> GSHMAKYTREDIEKLVKEENVKYIRLQFTDILGTIKNVEIPVSQLGKALDNKVMFDGSSIEGFVRIEESDMYLYPDLNTFVIFPWTAEKGKVARFICDIYNPDGTPFEGDPRNNLKRILKEMEDLGFSDFNLGPEPEFFLFKLDEKGEPTLELNDKGGYFDLAPTDLGENC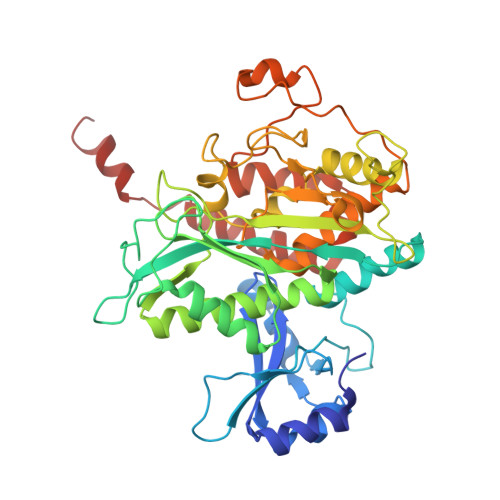RRDIVLELEEMGFEIEASHHEVAPGQHEIDFKYAGAVRSCDDIQTFKLVVKTIARKHGLHATFMPKPLFGVNGSGMHCNLSLFKNGVNAFFDENADLQLSETAKHFIAGIVKHATSFTAVTNPTVNSYKRLVPGYEAPCYVAWSAQNRSPLIRIPASRGISTRVEVRSVDPAANPYLALSVLLAAGLDGIKNKLEAPAPIDRNIYVMSKEERMENGIVDLPATLAEALEEFKSNEVMVKALGEHLFEHFIEAKEIEWDMFRTQVHPWEREQYMSQY7-(trifluoromethyl)-3,4-dihydroquinoxalin-2(1H)-one | C9 H7 F3 N2 O | 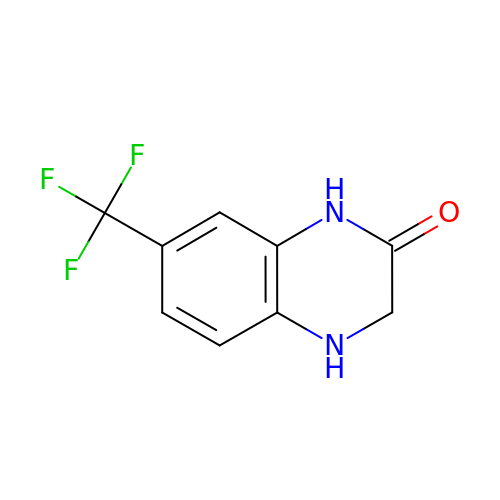DYBIQELZTJXUKA-UHFFFAOYSA-N>[4x]MEQLTKCEVFRELKDLKGYGGVSLPEWVCTTFHTSGYDTQAIVQNNDSTEYGLFQINN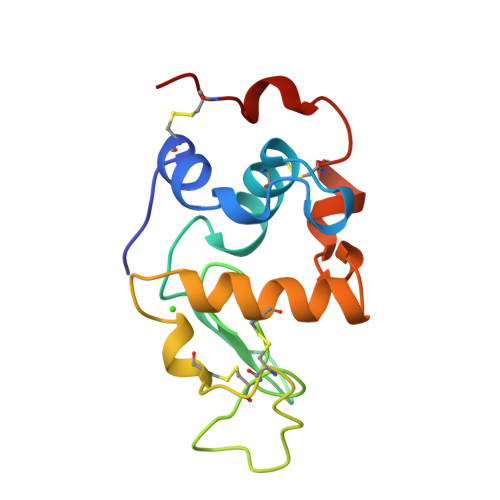KIWCKDDQNPHSSNICNISCDKFLDDDLTDDIVCVKKILDKVGINYWLAHKALCSEKLDQWLCEKL> MGSSHHHHHHMRVDGREKTELRHIHIHTNYL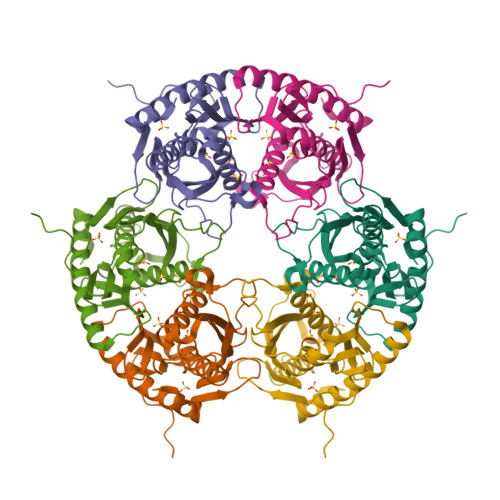KHPEGSVLIEVGDTKVICSATIEERVPPFMRGEGKGWVTAEYAMIPRATEQRTIRESSKGKVTGRTMEIQRLIGRALRAVVDLEALGERTVWIDCDVIQADGGTRTASITGAYVAMVLAFEKLLQAEKVSKIPVKDYLAATSVGIVEEQGVVLDLNYAEDSKADVDMNVIMTGKGQFVEVQGTGEEATFSRAQLNELLDAAEQGIFQLIDIQKEALGDIVSHIE>[4x]ATSWTMTAEQPDANYLTQNARQFA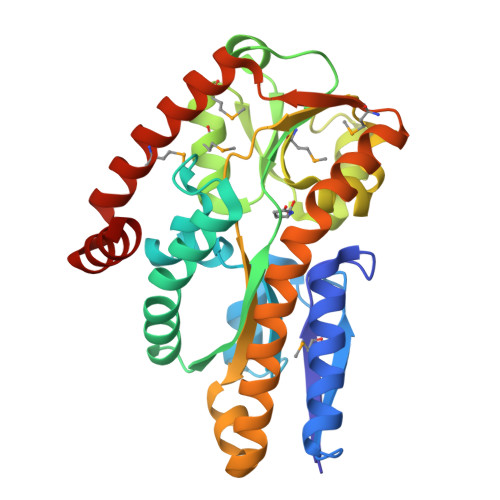DEVKAATAGALEIKVQSNSTLLKRPEVKRGVQQGVVQIGEVLVSALGNEDPLFEIDSVPFLASSFNESEKLWKATRPLLAQRLDKQGIVLVYGSPWPPQGIYTKKPVAALADLKGTRFRAYSASTSHMAALMGAVPTTVQTPEVPQAFSTGVIDAMLTSPATGVDSQAWDYVKYYYDAQAFIPQSFVIANKRAFQRLPAEVRQAVLDAGAKAEIRGWQTARAKTRELTDTLARNGMSVEPLPPQLAKELQAIGATMVSDWSKKAGADGQQLLDAYRK>[2x]MHHHHHHGSGSENLYFQGMETTDTKREEQEIEEKKAQEESKIEDVDKILNDILSISSECIQPDELRVKLLLKRKLICYDGFEPSGRMHIAQGLLKSIIVNKLTSNGCTFIFWIADWFAHLNNKMSGDLKKIKKVGSYFIEVWKSCGMNMENVQFLWASEEINKKPNEYWSLVLDISRSFNINRMKRCLKIMGRSEGEENYCSQILYPCMQCADIFFLNVDICQLGIDQRKVNMLAREYCDIKKIKKKPVILSHGMLPGLLEGQEKMSKSDENSAIFMDDSESDVNRKIKKAYCPPNVIENNPIYAYAKSIIFPSYNEFNLVRKEKNGGDKTYYTLQELEHDYVNGFIHPLDLKDNVAMYINKLLQPVRDHFQNNIEAKNLLNEIKKYKVTK

Like E1 enzymes, aminoacyl tRNA synthetases (aaRSs) are adenylate-forming enzymes (AFEs). They catalyze the transformation of amino acids into AMP conjugates, and then into aminoacyl-tRNAs, to supply protein synthesis. PfYRS is a Class I aaRS, characterized by a catalytic domain that adopts a Rossmann fold (residues 18–260) linked to a C-terminal domain (residues 261–370) that is involved in recognition of the anticodon stem of tRNATyr. PfYRS contains the two motifs characteristic of the catalytic domain of Class I (sub-class c) tRNA synthetases: “HIGH” and “KMSKS” (70HIAQ73 and 247KMSKS251 in PfYRS).

We identified adenosine 5′-sulfamate (AMS) as a broad specificity compound that hijacks a range of aaRSs; and ML901 as a specific reagent that hijacks a single aaRSs in the malaria parasite, Plasmodium falciparum, namely, tyrosine RS (PfYRS). The target enzyme catalyzes the formation of an inhibitory amino acid-sulfamate conjugate, via a reaction-hijacking mechanism. To confirm that recombinant PfYRS can generate the ML901-Tyr conjugate, we incubated PfYRS with substrates and ML901, then precipitated the tRNA and protein. To obtain crystals of ML901-Tyr-bound PfYRS, we incubated His-tagged PfYRS with tyrosine, ATP and ML901 in the presence of tRNA and then purified the complex using nickel affinity and gel filtration chromatography. In combination, these observations indicate different conformations of the KMSKS loop in individual monomers within the dimer. Potency and selectivity of ML901 for PfYRS thus appears to be associated with a stabilized loop over the active site.>MNPAAEAEFNILLATDSYKVTHYKQYPPNTSKVYSYFECREKKTENSKLRKVKYEETVFYGLQYILNKYLKGKVVTKEKIQEAKDVYKEHFQDDVFNEKGWNYILEKYDGHLPIEIKAVPEGFVIPRGNVLFTVENTDPECYWLTNWIETILVQSWYPITVATNSREQKKILAKYLLETSGNLDGLEYKLHDFGYRGVSSQETAGIGASAHLVNFKGTDTVAGLALIKKYYGTKDPVPGYSVPAAEHSTITAWGKDHEKDAFEHIVTQFSSVPVSVVSDSYDIYNACEKIWGEDLRHLIVSRSTQAPLIIRPDSGNPLDTVLKVLEILGKKFPVT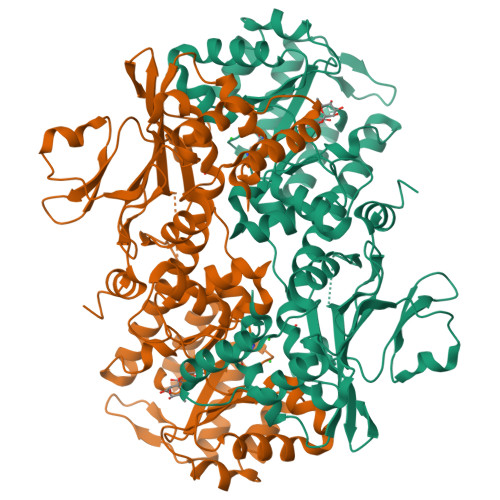ENSKGYKLLPPYLRVIQGDGVDINTLQEIVEGMKQKMWSIENIAFGSGGGLLQKLTRDLLNCSFKCSYVVTNGLGINVFKDPVADPNKRSKKGRLSLHRTPAGNFVTLEEGKGDLEEYGQDLLHTVFKNGKVTKSYSFDEIRKNAQLNIELEAAHHLEHHHHHH[2x]AusIA is a relatively rare α5/5-conotoxin isolated from the venom of Conus australis. Classical α-conotoxins are characterised by a CICII-Xm-CIII-Xn-CIV framework forming three possible disulfide connectivities: globular (I–III, II–IV), ribbon (I–IV, II–III) and bead (I–II, III–IV). α-Conotoxin AusIA is equipotent in the native globular and ribbon conformations in contrast to most other α-conotoxins where the globular isomer is more potent. In this paper, we present the co-crystal structure of gAusIA and rAusIA with Ls-AChBP that allowed us to understand the structural determinants underlying the equipotency at α7 nAChRs of two conformations.

The crystal structure of Ls-AChBP in complex with gAusIA and rAusIA were solved at 2.60 Å and 2.46 Å, respectively, using molecular replacement. The asymmetric unit contained one turbine-like pentamer and only one binding pocket was occupied by either gAusIA or rAusIA, possibly influenced by crystal packing. The C-loop was displaced outward by 10.3 ± 0.34 Å in the occupied binding interface, which is comparable to previous co-crystal structures of bound α-conotoxins (based on the measurement between Cys187 Cα atom in the complex with HEPES/Ls-AChBP structure), while the C-loops of other binding interfaces remained in a closed conformation. In this orientation, the first disulfide bond (CysI-CysIII for gAusIA and CysII-CysIII for rAusIA) packs against the C-loop vicinal disulfide bond with the central helix (residue 6–14) of both AusIA isomers protruding into the binding site in both complexes, forming an interacting core with the binding interface. While the electron density for both disulfide bonds of gAusIA is apparent, well-defined electron density is only presented for the CysII-CysIII disulfide bond of rAusIA. Despite this overlap, the second disulfide bond of rAusIA undergoes larger conformational fluctuations compared to gAusIA, as suggested from the ambiguous electron density of the second disulfide bond in rAusIA. Despite this difference in rigidity, the extent and nature of the pair-wise interactions contributed by gAusIA and rAusIA are similar. Similarly Arg5 in rAusIA also shows a degree of structural flexibility and no well-defined secondary structural units, allowing it to bind in a similar manner to the globular fold, explaining their equipotency. Meanwhile, rAusIA contacts are closer to Leu109, Gln115 and Leu119 compared to gAusIA, allowing stronger hydrophobic interactions that might be expected to compensate for the loss of the water-mediated hydrogen bonding.

>LDRADILYNIRQTSRPDVIPTQRDRPVAVSVSLKFINILEVNEITNEVDVVFWQQTTWSDRTLAWNSSHSPDQVSVPISSLWVPDLAAYNAISKPEVLTPQLARVVSDGEVLYMPSIRQRFSCDVSGVDTESGATCRIKIGSWTHHSREISVDPTTENSDDSEYFSQYSRFEILDVTQKKNSVTYSCCPEAYEDVEVSLNFRKKG[5x];> SCCARNPACRHNHPCV(9Z,11E,13S,15Z)-13-hydroxyoctadeca-9,11,15-trienoic 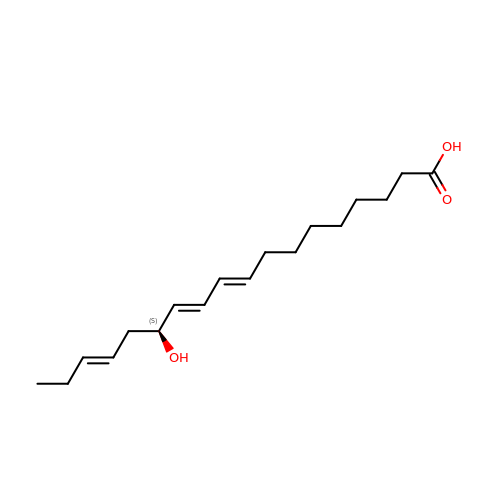acid | C18 H30 O3 | KLLGGGQNRTVBSU-FQSPHKRJSA-N> GARRFLCGVVEGFYGRPWVMEQRKELFRRLQKWELNTYLYAPKDDYKHRMFWREMYSVEEAEQLMTLISAAREYEIEFIYAISPGLDITFSNPKEVSTLKRKLDQVSQFGCRSFALLFDDIDHNMCAADKEVFSSFAHAQVSITNEIYQYLGEPETFLFCPTEYCGTFCYPNVSQSPYLRTVGEKLLPGIEVLWTGPKVVSKEIPVESIEEVSKIIKRAPVIWDNIHANDYDQKRLFLGPYKGRSTELIPRLKGVLTNPNCEFEANYVAIHTLATWYK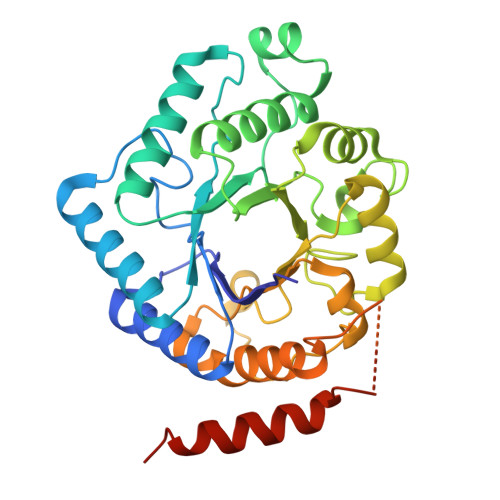SNMNGVRKDVVMTDSEDSTVSIQIKLENEGSDEDIETDVLYSPQMALKLALTEWLQEFGVPHQYSSR>MAQVQPWVDED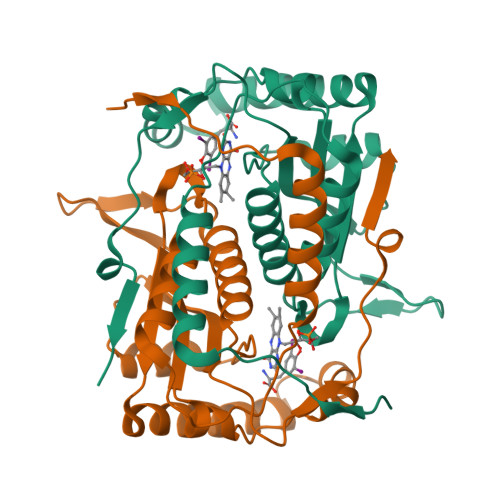LKDSTEDLQVEEDAEEWQEAEESVEHIPFSHTRYPEQEMRMRSQEFYELLNKRRSVRFISSEHVPMEVIENVIKAAGTAPSGAHTEPWTFVVVKDPDMKHKIREIIEEEEEINYMKRMGKRWVTDLKKLRTNWIKEYLDTAPVLILIFKQVHGFAANGKKKVHYYNEISVSIACGLLLAALQNAGLVTVTTTPLNCGPRLRVLLGRPSHEKLLVLLPVGYPSRDATVPDLKRKALDQIMVTVHHHHHH[8x]> MMNEKILIVDDQ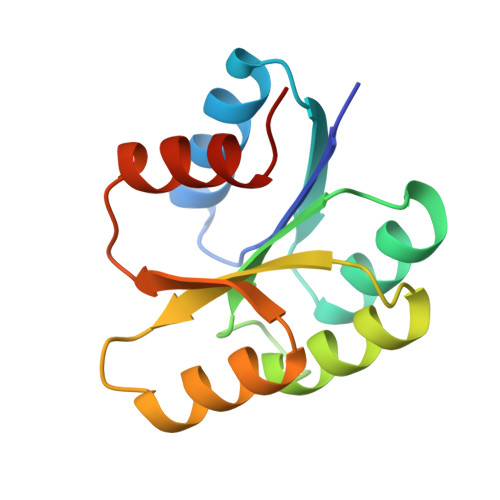YGIRILLNEVFNKEGYQTFQAANGLQALDIVTKERPDLVLLDMKIPGMDGIEILKRMKVIDENIRVIIMTAYGELDMIQESKELGALTHFAKPFDIDEIRDAVKKYLPLKSN>MKIQMRNKKVLSFLTLTAIVSQALVYPVYAQTSTSNHSNKKKEIVNEDILPNNGLMGYYFTDEHFKDLKLMAPIKDGNLKFEEKKVDKLLDKDKSDVKSIRWTGRIIPSKDGEYTLSTDRDDVLMQVNTESTISNTLKVNMKKGKEYKVRIELQDKNLGSIDNLSSPNLYWELDGMKKIIPEENLFLRDYSNIEKDDPFIPNNNFFDPKLMSDWEDEDLDTDNDNIPDSYERNGYTIKDLIA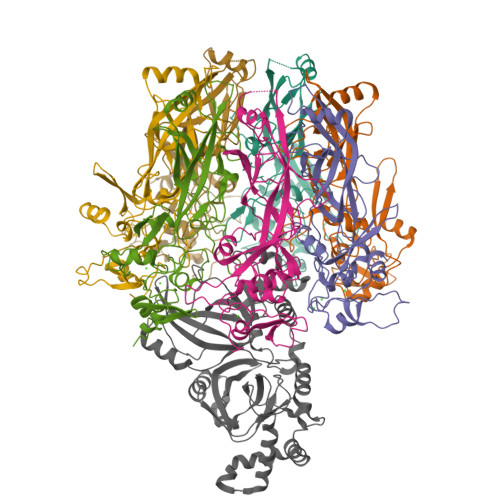VKWEDSFAEQGYKKYVSNYLESNTAGDPYTDYEKASGSFDKAIKTEARDPLVAAYPIVGVGMEKLIISTNEHASTDQGKTVSRATTNSKTESNTAGVSVNVGYQNGFTANVTTNYSHTTDNSTAVQDSNGESWNTGLSINKGESAYINANVRYYNTGTAPMYKVTPTTNLVLDGDTLSTIKAQENQIGNNLSPGDTYPKKGLSPLALNTMDQFSSRLIPINYDQLKKLDAGKQIKLETTQVSGNFGTKNSSGQIVTEGNSWSDYISQIDSISASIILDTENESYERRVTAKNLQDPEDKTPELTIGEAIEKAFGATKKDGLLYFNDIPIDESCVELIFDDNTANKIKDSLKTLSDKKIYNVKLERGMNILIKTPTYFTNFDDYNNYPSTWSNVNTTNQDGLQGSANKLNGETKIKIPMSELKPYKRYVFSGYSKDPLTSNSIIVKIKAKEEKTDYLVPEQGYTKFSYEFETTEKDSSNIEITLIGSGTTYLDNLSITELNSTPEILDEPEVKIPTDQEIMDAHKIYFADLNFNPSTGNTYINGMYFAPTQTNKEALDYIQKYRVEATLQYSGFKDIGTKDKEMRNYLGDPNQPKTNYVNLRSYFTGGENIMTYKKLRIYAITPDDRELLVLSVD[7x];> MKKFRKHKRISNCISILLILYLTLGGLLPNNIYAQDLQSYSEKVCNTTYKAPIERPEDFLKDKEKAKEWERKEAERIEQKLERSEKEALESYKKDSVEISKYSQTRNYFYDYQIEANSREKEYKELRNAISKNKIDKPMYVYYFESPEKFAFNKVIRTENQNEISLEKFNEFKETIQNKLFKQDGFKDISLYEPGKGDEKPTPLLMHLKLPRNTGMLPYTNTNNVSTLIEQGYSIKIDKIVRIVIDGKHYIKAEASVVSSLDFKDDVSKGDSWGKANYNDWSNKLTPNELADVNDYMRGGYTAINNYLISNGPVNNPNPELDSKITNIENALKREPIPTNLTVYRRSGPQEFGLTLTSPEYDFNKLENIDAFKSKWEGQALSYPNFISTSIGSVNMSAFAKRKIVLRITIPKGSPGAYLSAIPGYAGEYEVLLNHGSKFKINKIDSYKDGTITKLIVDATLIP>[2x]GSMVLNGYWGYQEFLDEFPEQRNLTNALSEAVRAQPVPLSKPTQRPIKISVVYPGQQVSDYWVRNIASFEKRLYKLNINYQLNQVFTRPNADIKQQSLSLMEALKSKSDYLIFTLDTTRHRKFVEHVLDSTNTKLILQNITTPVREWDKHQPFLYVGFDHAEGSRELATEFGKFFPKHTYYSVLYFSEGYISDVRGDTFIHQVNRDNNFELQSAYYTKATKQSGYDAAKASLAKHPDV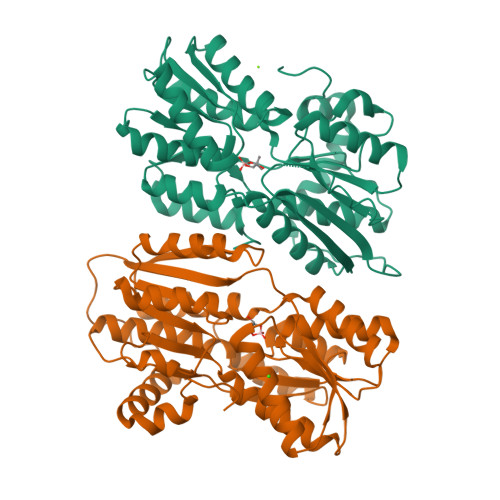DFIYACSTDVALGAVDALAELGREDIMINGWGGGSAELDAIQKGDLDITVMRMNDDTGIAMAEAIKWDLEDKPVPTVYSGDFEIVTKADSPERIEALKKRAFRYSDN>[2x]SNAVDICNHALLVGYGRVGSLLGEKLLASDIPLV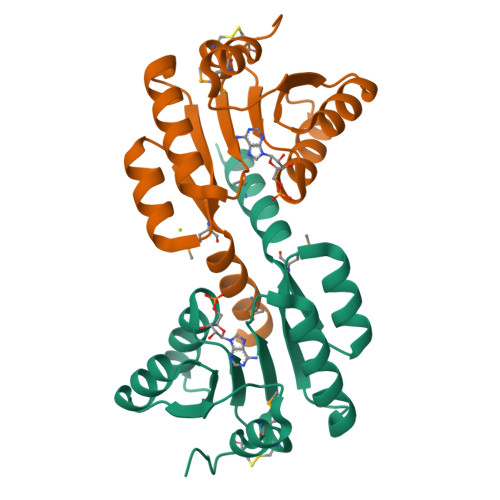VIETSRTRVDELRERGVRAVLGNAANEEIMQLAHLECAKWLILTIPNGYEAGEIVASARAKNPDIEIIARAHYDDEVAYITERGANQVVMGEREIARTMLELLETP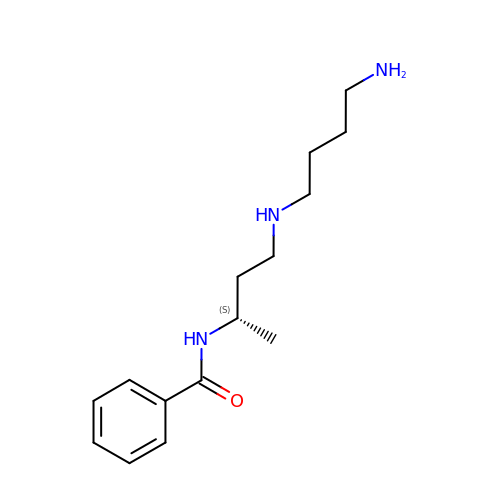N-{(1S)-3-[(4-aminobutyl)amino]-1-methylpropyl}benzamide | C15 H25 N3 O | UWDXTOVSVLCTLF-ZDUSSCGKSA-N>[3x]EAEAYVKSEWACPEGFTPKAGLNTDFPSDGKKRAFVVVPPKDSAGGAPVWVPMVGTVEATNWNLNVPRSGNNAKLAEHGYMVISPVRQCAEQDPNLGAGACNGVGKDGWTWNPWNDGRAPDASGDKYKTDAGDDVRFLEAMVRCVGTKWKLDRKRLFLGGISAGGTMTNRALLFDSEFWAGGMPISGEWYSTKDDGSTVPFQETR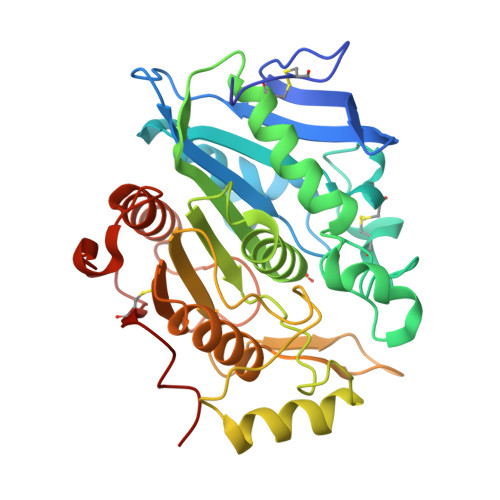KMVAAAPAKIWQGRVGPYPLPSKLDPMVVITVWGGEKDLWDCGPPLGLCSDYRPTTQASSNYFSSISNVVHVACSATHGHMWPQVNTDAFNLWALNTMASHPKGSSPKDFKLTAPPEGYSCKIGRFTDHYK> MGDDLLLKLLELLVEQARVSAEFARRQGDEKMLEEVARKAE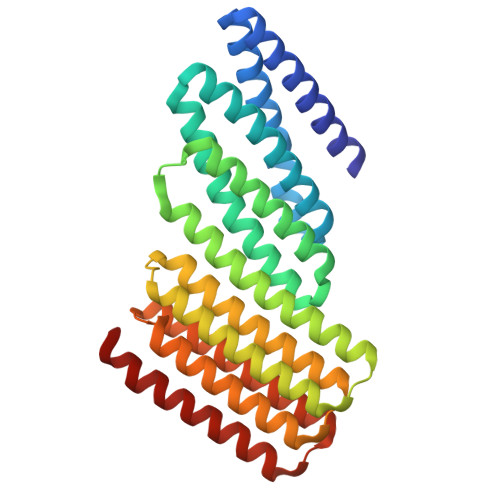EVARKAESIARKARKEGNLELALKALEILVRAAHVLAEIARERGNEELQKKAHKLAKEALRQVIEIAIRAIQEGNLELAIIALHISVRIAEVLLETRPDDREEIREQQAIFELLIAALEAAIRLEKLKEEGAPPEQIERVAEHGLERLKEIAKEISKEVDSPESKRIAYKIVAAAAEFLLKILAEGGATPEQLERVTEHALEVLKEVAKELADSPESGLAALAAIASLAKLGLEQLKEIGAPPEQQRRVTKAGIEAVREIYRYGRKLY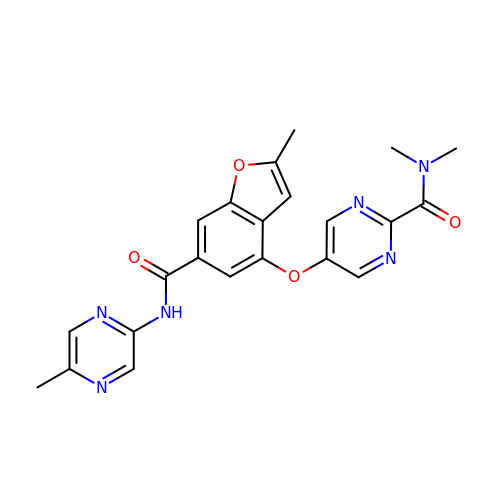N,N-dimethyl-5-({2-methyl-6-[(5-methylpyrazin-2-yl)carbamoyl]-1-benzofuran-4-yl}oxy)pyrimidine-2-carboxamide | C22 H20 N6 O4 | MASKQITXHVYVFL-UHFFFAOYSA-N>[2x]MLLEAIFHEAKGSYAYPISETQLRVRLRAKKGDVVRCEVLYADRYASPEEELAHALAGKAGSDERFDYFEALLECSTKRVKYVFLLTGPQGEAVYFGETGFSAERSKAGVFQYA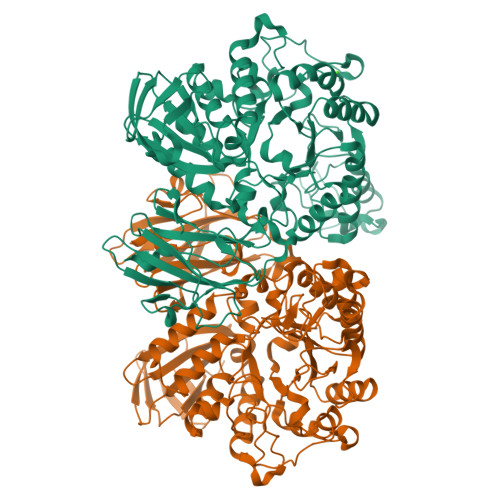YIHRSEVFTTPEWAKEAVIYQIFPERFANGDPSNDPPGTEQWAKDARPRHDSFYGGDLKGVIDRLPYLEELGVTALYFTPIFASPSHHKYDTADYLAIDPQFGDLPTFRRLVDEAHRRGIKIILDAVFNHAGDQFFAFRDVLQKGEQSRYKDWFFIEDFPVSKTSRTNYETFAVQVPAMPKLRTENPEVKEYLFDVARFWMEQGIDGWRLDVANEVDHAFWREFRRLVKSLNPDALIVGEIWHDASGWLMGDQFDSVMNYLFRESVIRFFATGEIHAERFDAELTRARMLYPEQAAQGLWNLLDSHDTERFLTSCGGNEAKFRLAVLFQMTYLGTPLIYYGDEIGMAGATDPDCKRPMIWEEKEQNRGLFEFYKELIRLRHRLASLTRGNVRSWHADKQANLYAFVRTVQDQHVGVVLNNRGEKQTVLLQVPESGGKTWLDCLTGEEVHGKQGQLKLTLRPYQGMILWNGR> MVGALLLASCKQAEEPKVAEKKAPVKVILVEAQIPPKPVKPPLPPLFSDIERRTFQFFWDTTNELNGLSPDRFPSRPFASIASVGFALTAYPIGIENGWVSRNQAIDRTLTTLKFFRDAPMGPQRTGKAGYKGFYYHFLDMQQGNRYDSWVELSSVDTALLMMGVLFTQSYYDGDDPREKEIRQIADTLYKRVDWRWLQQRAPLISMGWFPESGFIDHDWMGYNQAMMLYILALGSPTHGVEPDAWTVWTRTYNNDWGVYQGQEYLSFGPMFGHQYSHVWIDFRDIQDQYMRERGIDYFLNSRRATLAQRDYAIDNPMKWKDYGENVWGLTAGDGPQNTSQEYRGEQRQFRHYSSRGAGLRENFDDGTIAPTAAISSIVFAPEVVIPATEEMHKRYGDFLYSSYGFLDSFNPSFNYDIPLKTGRMVPDRGWVASDYIAIDQGPILAMIANYQNEFVWNVMKKNAYIRTGLERAGFTGGWLTPDGEPQPLPKKDEQAAAARALGMAESRAAAAQAQQDPSQRQHSSQRPKPELEHHHHHH

β‐1,2‐Glucans are natural glucose polymers produced by bacteria and play important physiological roles, including as symbiotic or pathogenic factors and in osmoregulation. Glycoside hydrolase (GH) families related to β‐1,2‐glucan metabolism (GH144, GH162, and GH189) have recently been created by identification of two β‐1,2‐glucanases and a β‐1,2‐glucanotransferase, respectively. Structural analysis of the proteins in Groups 1–4 revealed that they possess (α/α)6‐barrel folds similar to those of GH144, GH162, and GH189 enzymes. Overall, phylogenetic, biochemical, and structural analyses revealed that Groups 1–3 are new GH families, GH192, GH193, and GH194, respectively, and that the three families belong to clan GH‐S (clan GH, classification based on structural similarity) as GH144 and GH162.

GH144 protein from Xanthomonas campestris pv. campestris (XcSGL) was also used (Section 4). Because hydrolytic activities toward β‐1,2‐glucans were detected for PgSGL1, PgSGL2, PgSGL3, EeSGL1, SkSGLc, and XcSGL, the general properties of these enzymes were investigated using β‐1,2‐glucan alditols (see Section 4 for details) as substrates. While many of the enzymes showed optimal pH values around neutral pH, the optimal pH values of PgSGL3 and XcSGL were 8.5 and 5.0, respectively, which suggests that the optimal pH value varied within the SGL clan. XcSGL can be regarded as an SGL because of its narrow specificity for β‐1,2‐glucans and a similar level of specific activity toward β‐1,2‐glucans as the other SGLs. Comparison of spatial positions of predicted acidic catalytic residues suggested that Groups 1–3 and GH144 had the same reaction mechanism.>MRFIHALLLAGIAHSAYASEKLTFKTDLEKLEREKAAQIGVAIVDPQGEIVAGHRMAQRFAMGSTFKFPLAALVFERIDSGTERGDRKLSYGPDMIVEWSPATERFLASGHMTVLEAAQAAVQLSDNGATNL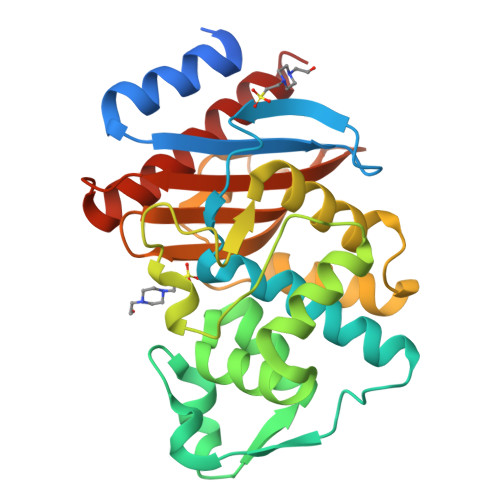LLREIGGPAAMTQYFRKIGDSVSRLDRKEPEMSDNTPGDLRDTTTPIAMARTVAKVLYGGALTSTSTHTIERWLIGNQTGDATLRAGFPKDWVVGEKTGTCANGGRNDIGFFKAQERDYAVAVYTTAPKLSAVERDELVASVGQVITQLILSTDK[2x]>RRVVVTGLGMVTPLGRGVETTWRRLIDGECGIRGLTLDDLKMKSFDEETKLYTFDQLSSKVAAFVPYGSNPGEFDEALWLNSKAVANFIGYAVCAADEALRDAEWLPTEEEEKERTGVSIGGGIGSICDIVEAAQLICEKRLRRLSPFFIPKILVNMASGHVSMKYGFQGPNHAAVTACATGAHSIGDATRMIQFGDADVMVAGGTESSIDALSVAGFSRSRALSTKFNSSPQEASRPFDCDRDGFVIGEGSGVIVLEEYEHAKRRGAKIYAELCGYGMSGDAHHITQPPEDGKGAVLA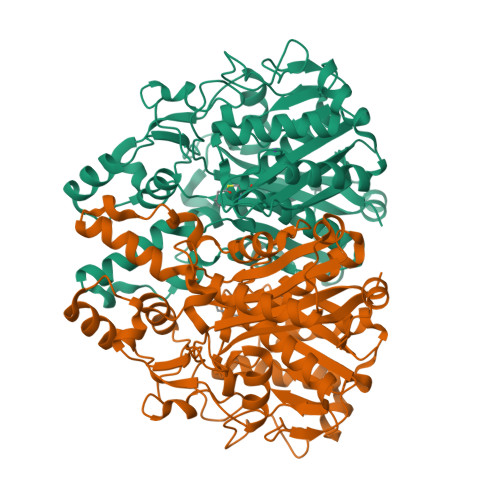MTRALRQSGLCPNQIDYVNAHATSTPIGDAVEARAIKTVFSEHATSGTLAFSSTKGATGHLLGAAGAVEAIFSILAIHHGVAPMTLNVKNPDPIFDKRFMPLTTSKKMLVRTAMSNSFGFGGTNASLLFASI[2x]>[2x]MNDSQTMLILLCNVNIYAPNPLGIKDVLIAGNKIAAIYDHGQGEITIPKQWPVKVINFDGAILTPGFIDSHAHITGGGGQAGFATQVPPVGLTEFTHAGVTTVVGLLGT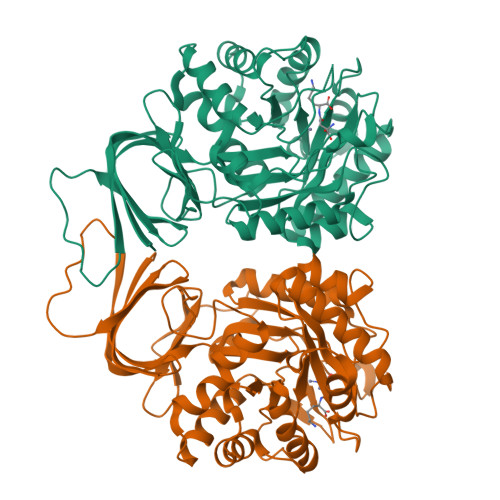DDTTRSTENLLSRVYGLREEGLSAYCWTGGYHFPLTTITGSAKSDIAFLEPVIGIGEFAISDHRSSQPTFEEVIRLASETHVAGLITGKAGVIHFHLGDGERRLELIERAIRETELPARVFNPTHVNRNKPLFEDSCKLLSKGCHIDLTAFPAGTAQPGWEACDAIEMAVERQLPLEQITLSSDGGGCLPCFDPQGELQHMDFGRASTLGETLVATLNKGLSLETVLPMLTSNVANILRFKNKGQIAVGFDADLLVMNEKYEITDVMAQGVWHKQNNQTMIKGTFE> SSLDDKPQFPGASAEFIDKLEFIQPNVISGIPIYRVMDRQGQIINPSEDPHLPKEKVLKLYKSMTLLNTMDRILYESQRQGRISFYMTNYGEEGTHVGSAAALDNTDLVFGAYREAGVLMYRDYPLELFMAQCYGNISDLGKGRQMPVHYGCKERHFVTISSPLATQIPQAVGAAYAAKRANANRVVICYFGEGAASEGDAHAGFNFAATLECPIIFFCRNNGYAISTPTSEQYRGDGIAARGPGYGIMSIRVDGNDVFAVYNATKEARRRAVAENQPFLIEAMTYRIGHASTSDDSSAFRSVDEVNYWDKQDHPISRLRHYLLSQGWWDEEQEKAWRKQSRRKVMEAFEQAERKPKPNPNLLFSDVYQEMPAQLRKQQESLARHLQTYGEHYPLDHFDK;> VAHFTFQPDPEPREYGQTQKMNLFQSVTSALDNSLAKDPTAVIFGEDVAFGGVFRCTVGLRDKYGKDRVFNTPLCEQGIVGFGIGIAVTGATAIAEIQFADYIFPAFDQIVNEAAKYRYRSGDLFNCGSLTIRSPWGCVGHGALYHSQSPEAFFAHCPGIKVVIPRSPFQAKGLLLSCIEDKNPCIF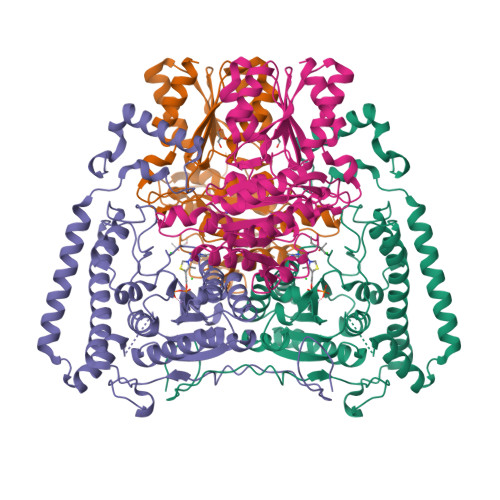FEPKILYRAAAEEVPIEPYNIPLSQAEVIQEGSDVTLVAWGTQVHVIREVASMAKEKLGVSCEVIDLRTIIPWDVDTICKSVIKTGRLLISHEAPLTGGFASEISSTVQEECFLNLEAPISRVCGYDTPFPHIFEPFYIPDKWKCYDALRKMINY>[2x]NDETKALKELYGPVDPTFLHRFYSLKAAVHGWKMVVCDKVRSLKLSDNNCYLNAVIMTLDLLKDIKFVIPALQHAFMKHKGGDSTDFIALIMAYGNCTFGAPDDASRLLHTVLAKAELCCSARMVWREWCNVCGIKDVVLQGLKACCYVGVQTVEDLRARMTYVCQCGGERHRQLVEHTTPWLLLS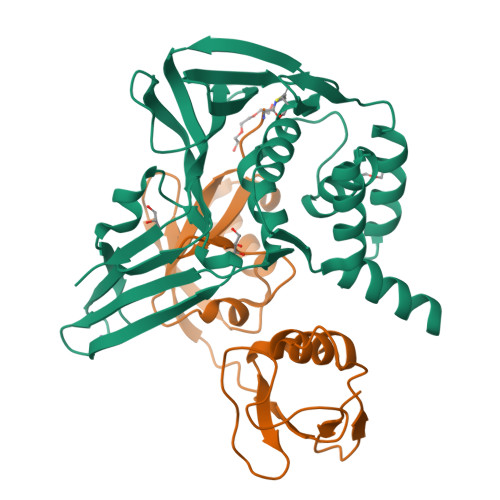GTPNEKLVTTSTAPDFVAFNVFQGIETAVGHYVHARLKGGLILKFDSGTVSKTSDWKCKVTDVLFPGQKYSSD;>MGWDLTVKMLAGNEFQVSLSSSMSVSELKAQITQKIGVHAFQQRLAVHPSGVALQDRVPLASQGLGPGSTVLLVVDKSDEPLSILVRNNKGRSSTYEVRLTQTVAHLKQQVSGLEGVQDDLFWLTFEGKPLEDQLPLGEYGLKPLSTVFMNLRLRG[2x]>[3x]AAYSQGGGKKKVCYYYDGDIGNYYYGQGHPMKPHRIRMTHNLLLNYGLYRKMEIYRPHKATAEEMTKYHSDEYIKFLRSIRPDNMSEYSKQMQRFNVGEDCPVFDGLFEFCQLSTGGSVAGAVKLNRQQTDMAVNWAGGLHHAKKSEASGFCYVNDIVLAILELLKYHQRVLYIDIDIHHGDGVEEAFYTTDRVM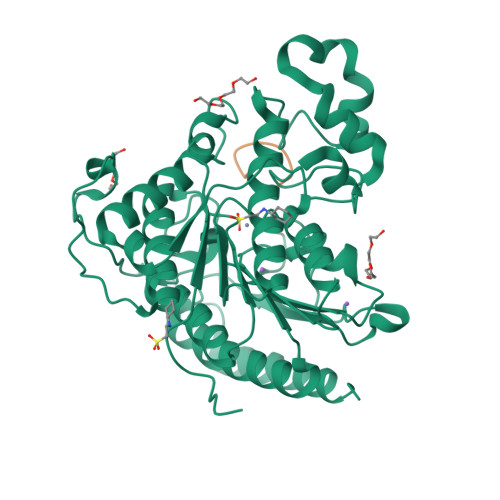TVSFHKYGEYFPGTGDLRDIGAGKGKYYAVNFPMRDGIDDESYGQIFKPIISKVMEMYQPSAVVLQCGADSLSGDRLGCFNLTVKGHAKCVEVVKTFNLPLLMLGGGGYTIRNVARCWTYETAVALDCEIPNELPYNDYFEYFGPDFKLHISPSNMTNQNTPEYMEKIKQRLFENLRMLPHAPGVQMQAI;>XNPEQKWG[3x]>[2x]MKITDLELHAVGIPRHTGFVNKHVIVKIHTDEGLTGIGEMSDFSHLPLYSVDLHDLKQGLLSI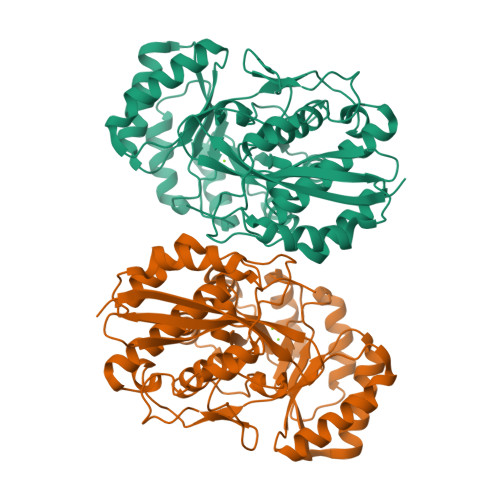LLGQNPFDLMKINKELTDNFPETMYYYEKGSFIRNGIDNALHDLCAKYLDISVSDFLGGRVKEKIKVCYPIFRHRFSEEVESNLDVVRQKLEQGFDVFRLYVGKNLDADEEFLSRVKEEFGSRVRIKSYDFSHLLNWKDAHRAIKRLTKYDLGLEMIESPAPRNDFDGLYQLRLKTDYPISEHVWSFKQQQEMIKKDAIDIFNISPVFIGGLTSAKKAAYAAEVASKDVVLGTTQELSVGTAAMAHLGCSLTNINHTSDPTGPELYVGDVVKNRVTYKDGYLYAPDRSVKGLGIELDESLLAKYQVPDLSWDNVTVHQLQDRTADTKS2,3-BIS-BENZO[1,3]DIOXOL-5-YLMETHYL-SUCCINIC 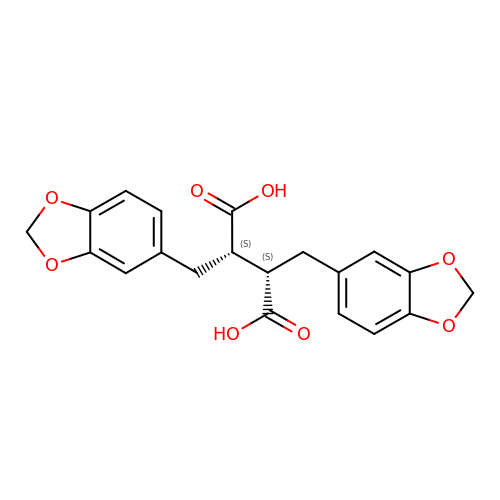ACID | C20 H18 O8 | FFYBYVPVYLMLAR-KBPBESRZSA-N> RSMSEVITI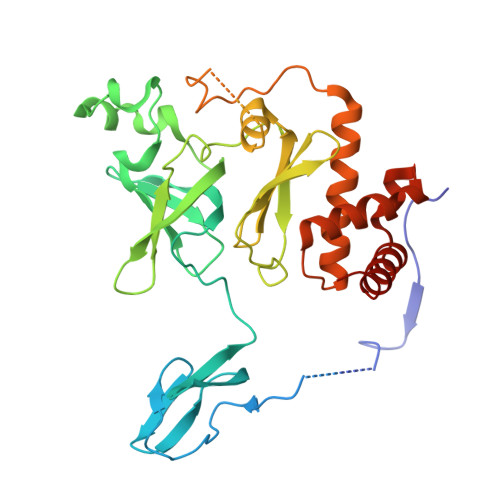TKRNGAFQNSSNLSYNNTGISDDENDEEDIYMHDVNSASKSESDSQIVTPGELVTDDPIWMRGHGTYFLDNMTYSSVAGTVSRVNRLLSVIPLKGRYAPETGDHVVGRIAEVGNKRWKVDIGGKQHAVLMLGSVNLPGGILRRKSESDELQMRSFLKEGDLLNAEVQSLFQDGSASLHTRSLKYGKLRNGMFCQVPSSLIVRAKNHTHNLPGNITVVLGVNGYIWLRKTSQMDLARDTPSANNSSSIKSTGPTGAVSLNPSITRLEEESSWQIYSDENDPSISNNIRQAICRYANVIKALAFCEIGITQQRIVSAYEASMVYSNVGELIEKNVMESIGSDILTAEKMRGNGN1,4-bis({2-[(2-hydroxyethyl)amino]ethyl}amino)anthracene-9,10-dione | C22 H28 N4 O4 | 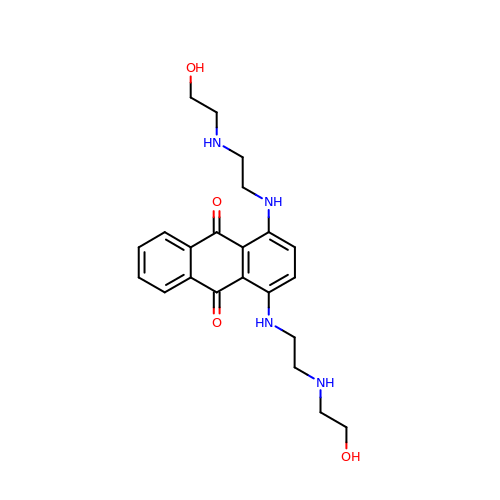FFGSXKJJVBXWCY-UHFFFAOYSA-N>[2x]AGFQLNEFSSSGLGRAYSGEGAIADDAGNVSRNPALITMFDRPTFSAGAVYIDPDVNISGTSPSGRSLKADNIAPTAWVPNMHFVAPINDQFGWGASITSNYGLATEFNDTYAGGSVGGTTDLETMNLNLSGAYRLNNAWSFGLGFNAVYARAKIERFAGDLGQLVAGQIMQSPAGQTQQGQALAATANGIDSNTKTAH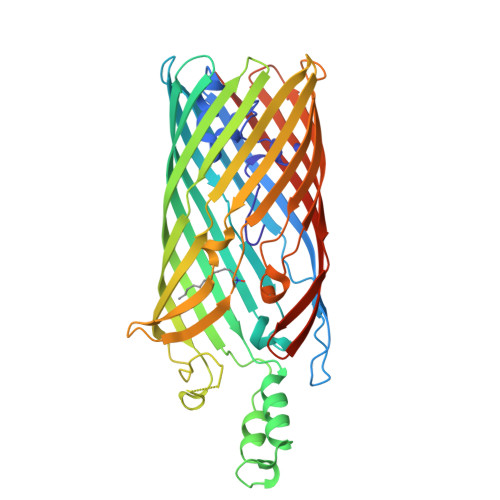LNGNQWGFGWNAEILYELDKNNRYALTYRSEVKIDFKGNYSSDLNRAFNNYGLPIPTATGGATQSGYLTLNLPEMWEVSGYNRVDPQWAIHYSLAYTSWSQFQQLKATSTSGDTLFQKHEGFKDAYRIALGTTYYYDDNWTFRTGIAFDDSPVPAQNRSISIPDQDRFWLSAGTTYAFNKDASVDVGVSYMHGQSVKINEGPYQFESEGKAWLFGTNFNYAFHHHHHH> MAEVVNGKLHLRFAIAPMRPTPSQTIKEFEPIFKYLADQLGATYEIVSPESWAAISVAMTNGHVDVGWLGPWGYVLSNKKA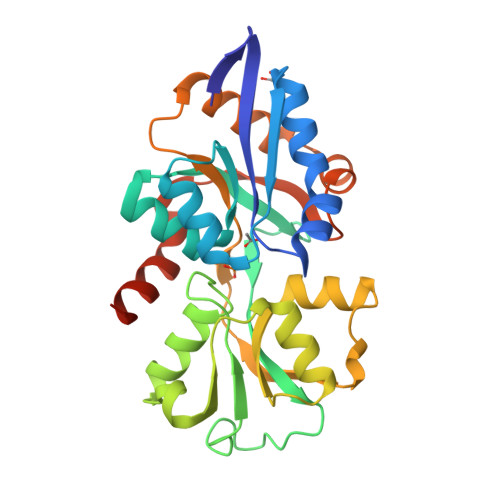GTEVLATVKYRGEPFYKALIVGRADLPIKKWPEDAKGLKLSLSDQGNTSGWLIPMAYFKSIGIDPASYFEYREGATFGQNESQIQHGLIDLGSDMDRGRNGMIEAGQIDPSKSKIVWESSKLPNAAISVPKDFDPALKARITEILTSLSEEKAQSLMGSGYNGFVKAKHSDYKVIEDAGRILGKLLEHHHHHH3-(3-{[3-(4-carboxyphenoxy)phenyl]methoxy}phenyl)-1H-indole-2-carboxylic acid | C29 H21 N O6 | 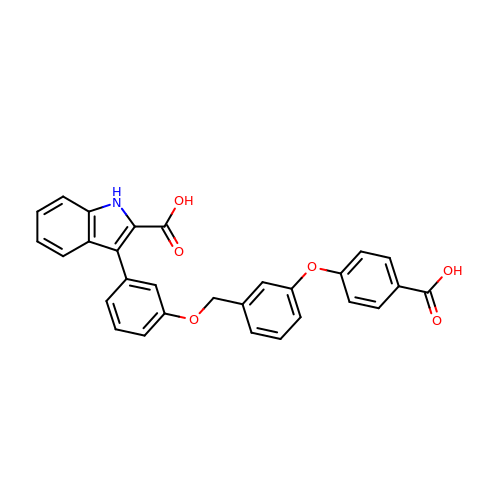PSBGQCWQSZIAEZ-UHFFFAOYSA-N>[2x]EFADAPIDTKTTMDYITPSFANKAGKPKACYVTLVRNKELKGLLSSIKYVENKINKKFPYPWVFLNDEPFTEEFKEAVTKAVSSEVKFGILPKEHWSYPEWINQTKAAEIRADAATKYIYGGSESYRHMCRYQSGFFWRHELLEEYDWYWRVEPDIKLYCDINYDVFKWMQENEKVYGFTVSIHEYEVTIPTLWQTSMDFIKKNPEYLDENNLM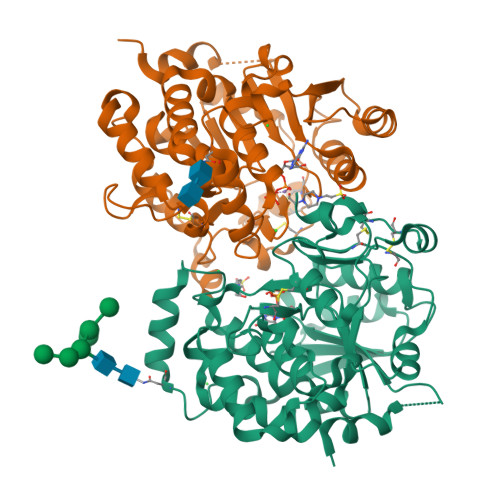SFLSNDNGKTYNLCHFWSNFEIANLNLWRSPAYREYFDTLDHQGGFFYERWGDAPVHSIAAALFLPKDKIHYFSDIGYHHPPYDNCPLDKEVYNSNNCECDQGNDFTFQGYSCGKEYYDAQGLVKPKNWKKFRE>[2x]SNAMDMYHTKILKAIESEDYISVRRRVLRQLVESLIYEGIITPARIEKEEQILFLIQGLDEDNKSVTYECYGRERITFGRISIDSLIVRVQDGKQEIQSVAQFLEEVFRVVNVEQTKLDSFIHELEQTIFKDTIAQYERCNKLKYTQKSYDELENHLIDGHPYHPSYKARIGFQYRDNFRYGYEFMRPIKLIWIAAHKKNATVGYENEVIYDKILKSEVGERKLEAYKERIHSMGCDPKQYLFIPVHPWQWENFIISNYAEDIQDKGIIYLGESADDYCAQQSMRTLRNVTNPKRPYVKVSLNILNTSTLRTLKPYSVASAPAISNWLSNVVSQDSY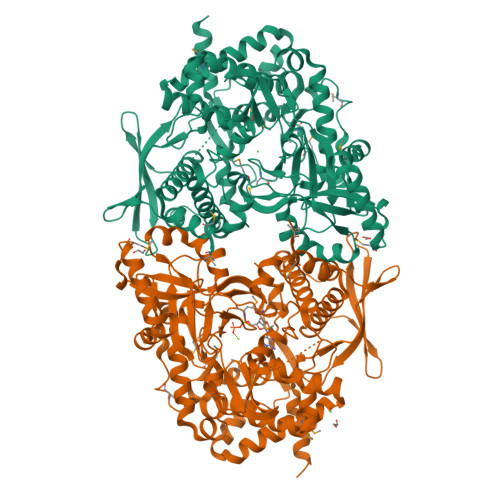LRDESRVILLKEFSSVMYDTNKKATYGSLGCIWRESVHHYLGEQEDAVPFNGLYAKEKDGTPIIDAWLNKYGIENWLRLLIQKAIIPVIHLVVEHGIALESHGQNMILVHKEGLPVRIALKDFHEGLEFYRPFLKEMNKCPDFTKMHKTYANGKMNDFFEMDRIECLQEMVLDALFLFNVGELAFVLADKYEWKEESFWMIVVEEIENHFRKYPHLKDRFESIQLYTPTFYAEQLTKRRLYIDVESLVHEVPNPLYRARQLNIQKSVATGGNYANCENLYFQ>[2x]SVDREEMIERFANFLREYTDEDGNPVYRGKITDLLTITPKRSVAIDWMHLNSFDSELAHEVIENPEEGISAAEDAIQIVLREDFQREDVGKIHARFYNLPETLMVKDIGAEHINKLIQVEGIVTRVGEIKPFQSFRIQDRPETLKGGEMPRFIDGILLDDIVDVALPGDRVIVTGILRVVLEKREKTPIFRKILEVNHIEPVSKEI

The Minichromosome Maintenance (MCM) complex forms an essential hexameric-ring helicase that unwinds DNA at the replication fork (1–3). MCM proteins have three conserved domains: an N-terminal domain (MCMN) that mediates the head-to-head interaction of the initial double-hexamer; a conserved AAA+ ATPase domain; and a short helix-turn-helix domain at the C-terminus. Crystal structures of the N-terminal domains of Methanobacterium thermautotrophicus (MtMCMN), Sulfolobus solfataricus (SsoMCMN) and Pyrococcus furiosis (PfMCMN) show a consistent hexameric ring structure with three subdomains: a helical subdomain-A, a Zn-binding subdomain-B and an OB-fold subdomain-C. The crystal structure of PfMCMN bound to single-stranded DNA (ssDNA) revealed that subdomain-C binds ssDNA in the plane of the hexameric ring via conserved residues defined as the MCM single-stranded DNA-binding motif (MSSB).

We designed the PfMCMN-ΔZFD construct to disrupt the short intersubunit antiparallel β-sheet interaction (P130 carbonyl–F240 amide and V132 amide–P238 carbonyl). Because these interactions exclusively involve main-chain atoms, they cannot be predictably disrupted by side-chain mutagenesis. Instead, we deleted residues 131–181, which deletes the Zn-binding B-subdomain. This deletion removes the V132 amide altogether and requires a different orientation for the P130 carbonyl to accommodate the tight β-hairpin needed to accommodate the deletion. We confirmed that the deletion indeed removed the potential for the short intersubunit β-sheet interaction by determining its crystal structure to 1.55 Å resolution. The structure shows that P130 adopts a cis-proline conformation in order to generate the tight β-hairpin of the deletion, and thus the carbonyl of this residue is no longer available to interact with a neighboring subunit. Notably, the MSSB residues of PfMCMN-ΔZFD are positioned very similar to those of PfMCMN-WT when bound to ssDNA. The PfMCMN-ΔZFD and PfMCMN-F179A mutants are exclusively monomeric at all concentrations tested. All of these mutants (PfMCMN-ΔZFD, PfMCMN-F179A and PfMCMN-βT) have wild-type MSSB motifs available for interaction with ssDNA, but no binding is observed.> MDPKAEGNGENITETAAGNVETSDFVNLKRQKREGVNSTGMSEIDMTGSQETPEHNMHGSPTHTDDLGPRLDADMLDSQSSHVSSSAQGNRSEVENELSNLFAKMALPGHDRRTDEYILVRQTGQDKFAGTTKCNLDHLPTKAEFNASCRLYRDGVGNYYPPPLAFERIDLPEQLAAQLHNLEPREQSKQCFQYKLEVWNRAHAEMGITGTDIFYQTDKNIKLDRNYKLRPEDRYIQTEKYGRREIQKRYEHQFQAGSLLPDILIKTPQNDIHFSYRFAGDAYANKRFEEFERAIKTKYGSDTEIKLKSKSGIMHDSKYLESWERGSA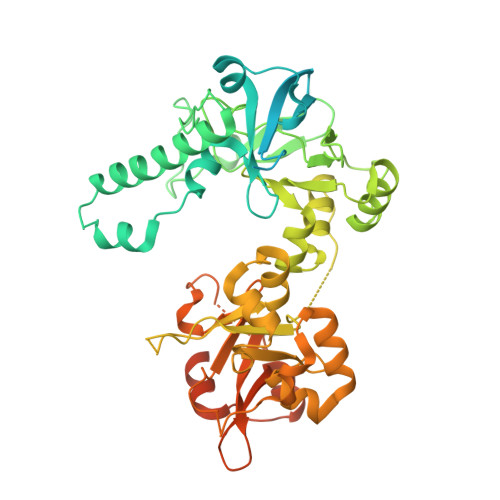DIRFAEFAGENRAHNKQFPAATVNMGRQPDGQGGMTRDRHVSVDYLLQNLPNSPWTQALKEGKLWDRVQVLARDGNRYMSPSRLEYSDPEHFTQLMDQVGLPVSMGRQSHANSVKFEQFDRQAAVIVADGPNLREVPDLSPEKLQQLSQKDVLIADRNEKGQRTGTYTNVVEYERLMMKLPSDAAQLLAEPSDRYSRAFVRPEPALPPISDSRRTYESRPRGPTVNSL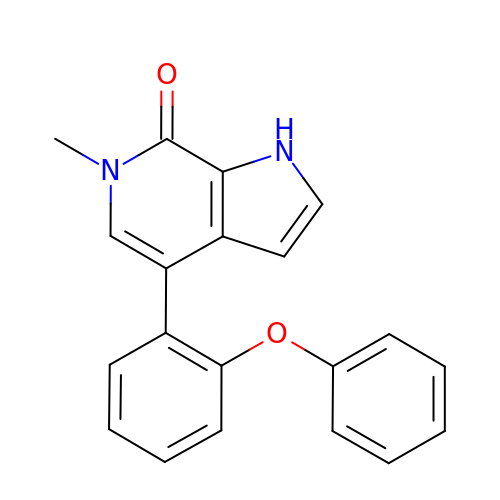6-methyl-4-(2-phenoxyphenyl)-1,6-dihydro-7H-pyrrolo[2,3-c]pyridin-7-one | C20 H16 N2 O2 | NUAFIMXCNWRSMX-UHFFFAOYSA-N N'-(3-bromophenyl)-4-fluoro-N-hydroxy-3-(trifluoromethyl)benzenecarboximidamide 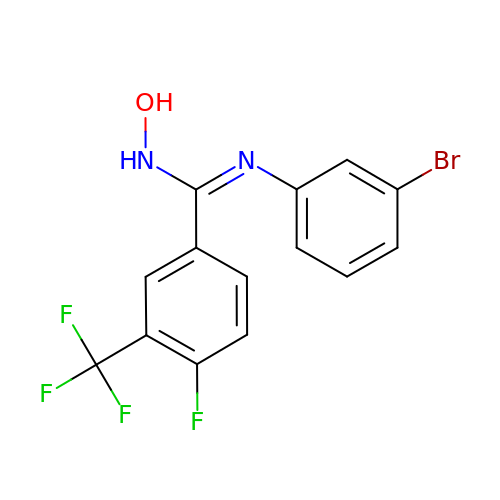| C14 H9 Br F4 N2 O | HYMULNGSTZFRLI-UHFFFAOYSA-N>[3x]MTKAVHTKHAPAAIGPYSQGIIVNNMFYSSGQIPLTPSGEMVNGDIKEQTHQVFS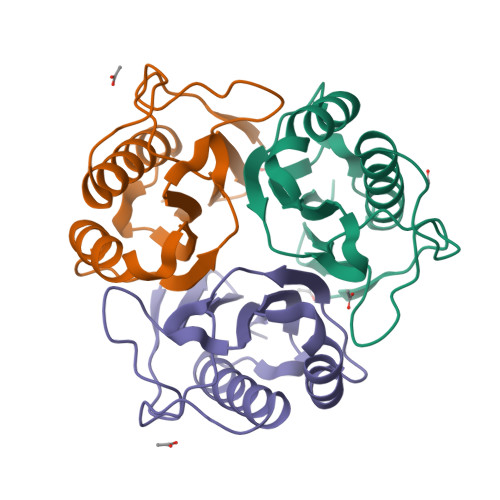NLKAVLEEAGASFETVVKATVFIADMEQFAEVNEVYGQYFDTHKPARSCVEVARLPKDALVEIEVIALVK>[2x]MSFLFSSRSSKTFKPKKNIPEGSHQYELLKHAEATLGSGNLRQAVMLPEGEDLNEWIAVNTVDFFNQINMLYGTITEFCTEASCPVMSAGPR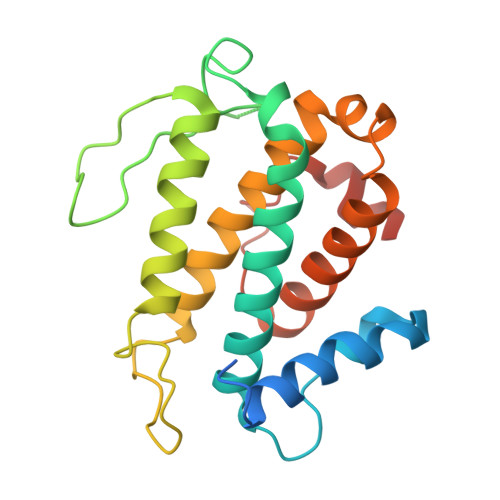YEYHWADGTNIKKPIKCSAPKYIDYLMTWVQDQLDDETLFPSKIGVPFPKNFMSVAKTILKRLFRVYAHIYHQHFDSVMQLEEEAHLNTSFKHFIFFVQEFNLIDRRELAPLQELIEKLGSKDR> VPHTLSTLKTADNRPASVYL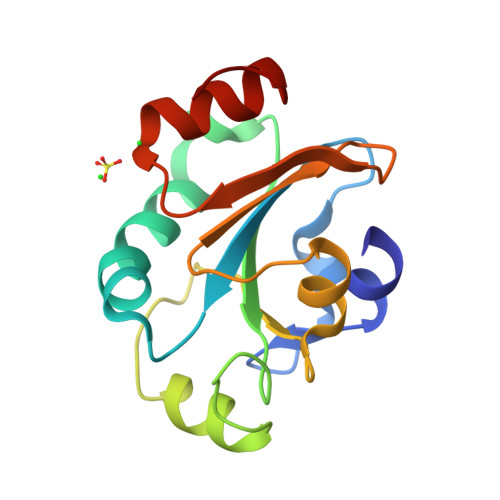KKDKPTLIKFWASWCPLCLSELGQTEKWAQDAKFSSANLITVASPGFLHEKKDGDFQKWYAGLNYPKLPVVTDNGGTIAQSLNISVYPSWALIGKDGDVQRIVKGSINEAQALALIRDPNADL> NTEIIKSFKNFILEFRLDSQFIYRDQLRNNILVKNYSLTVNMEHLIGYNEDIYKKLSDEPSDIIPLFETAITQVAKRISILSRAQSANNNDKDPENTSMDTDSLLLNSLPTFQLILNSNANQIPLRDLDSEHVSKIVRLSGIIISTSVLSSRATYLSIMCRNCRHTTSITINNFNSITGNTVSLPRSCLSTIESESSMANESNIGDESTKKNCGPDPYIIIHESSKFIDQQFLKLQEIPELVPVGEMPRNLTMTCDRYLTNKVIPGTRVTIVGIYSIYNSKNGAGSGRSGGGNGGSGVAIRTPYIKILGIQSDVETSSIWNSVTMFTEEEEEEFLQLSRNPKLYEILTNSIAPSIFGNEDIKKAIVCLLMGGSKKILPDGMRLRGDINVLLLGDPGTAKSQLLKFVEKVSPIAVYTSGKGSSAAGLTASVQRDPMTREFYLEGGAMVLADGGVVCIDEFDKMRDEDRV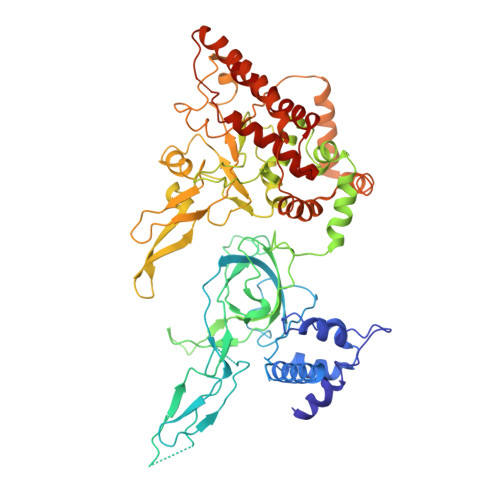AIHEAMEQQTISIAKAGITTVLNSRTSVLAAANPIYGRYDDLKSPGDNIDFQTTILSRFDMIFIVKDDHNEERDISIANHVINIHTGNANAMQNQQEENGSEISIEKMKRYITYCRLKCAPRLSPQAAEKLSSNFVTIRKQLLINELESTERSSIPITIRQLEAIIRITESLAKLELSPIAQERHVDEAIRLFQASTMDAAS>HHHHHHPVLLKSTETGQYLRINPDGTVDGTRDRSDPHIQF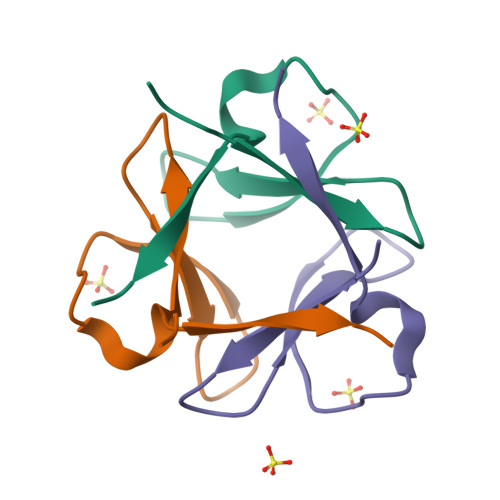QISPEGNG[3x]>SNAKDSIVNDDDDSTSEVDAISDSTNPSGSFPSVEYEVFLSFRGPDTREQFTDFLYQSLRRYKIHTFRDDDELLKGKEIGPNLL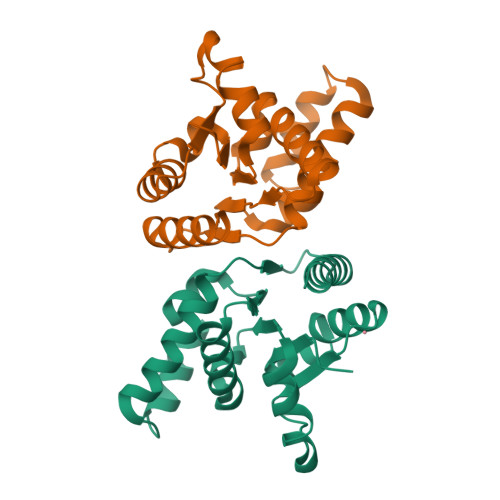RAIDQSKIYVPIISSGYADSKWCLMELAEIVRRQEEDPRRIILPIFYMVDPSDVRHQTGCYKKAFRKHANKFDGQTIQNWKDALKKVGDLKGWHIGKNDKQGAIADKVSADIWSHISKEN[2x]>MKLSARNQLAGKVVSIKEGAVNGIVVLDIGGGNQISSTISMDSIRELGLQVGSDAYAVIKATSVMIGIDDWSHPQFEK[6x]

Here, we characterized E. limosum Tub, a tungsten storage protein. Tub has a sub-nanomolar affinity for tungstate and contains a single TOBE domain first characterized in a molybdate storage protein. Crystal structures revealed Tub assembles as a hexamer composed of a trimer of dimers, capable of binding eight tungstate oxyanions at two distinct binding sites located at inter-subunit interfaces. Tub enables E. limosum to accumulate W and then supplies W for two tungstoenzymes needed for conversion of lactate to SCFAs.

The X-ray crystal structure of tungstate-bound rTub was determined at 1.85 Å resolution. It consists predominantly of β-strands (59.1%), where the C-terminal half of the β1, β2, and β3 form a three-stranded antiparallel β-sheet. The Tub dimer is formed by another three-stranded antiparallel β-sheet consisting of N-terminal half of β1, β4, and the β5′ from the neighboring monomer. There is also a short α-helix between β3 and β4 and a 310-helical segment between β4 and β5. Tub has eight tungstate binding sites, where two (type-1) lie at opposite poles of the hexamer with a cavity that is open to the surface. Tungstate binding involves H-bonding to the backbone of Ala20, Val21, and Asn22 from each of the three monomers along the threefold axis. The overall structure of the type-1 binding site is similar to that of the molybdate binding protein, ModG. The six type-2 binding sites in Tub are located at the interface of two adjacent monomers by non-crystallographic twofold symmetry producing two binding sites for every dimer. The type-2 sites are buried in the interior of the Tub hexamer with no direct connection to the solvent when tungstate is bound, which forms a complex H-bonding network involving the backbones of Arg6 and Ala61, and sidechains of Ser4 and Lys 60 from one monomer, and Ser40 backbone and sidechain from neighboring monomer. This binding site is very similar to that found in Mop and ModE.> SPIPVTIREHAGTWYSTLPDSTVPIYGKTPVAPANYMVGE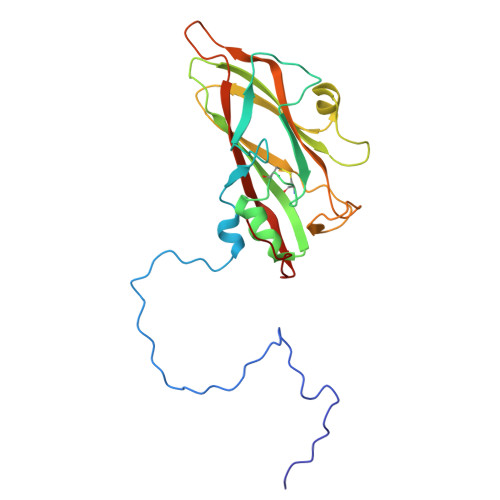YKDFLEIAQIPTFIGNKMPNAVPYIEASNTAVKTQPLAVYQVTLSCSCLANTFLAALSRNFAQYRGSLVYTFVFTGTAMMKGKFLIAYTPPGAGKPTSRDQAMQATYAIWDLGLNSSYSFTVPFISPTHFRMVGTDQANITNVDGWVTVWQLTPLTYPPGCPTSAKILTMVSAGKDFSLKMPISPAPWSPQ>[2x]GWLDLAPSTQVDTETSINVLSDIEFTLNGIYSTMQSSDAYSGRLVYYGDVTGDDMQAVSSTKRTGNYYRFNF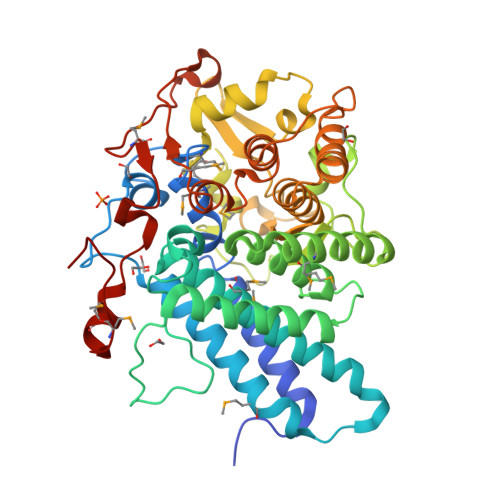TKDNGPSSHWSYLYSIIQNCNLILMNVDKLSIDEDETEYKNDLKGQALAIRGMALFDLTRIFGYPYLKDNGASLGVPIVKELSTIDSKPARNTVAECYTEIISDLKNSTELLSGDFNKGKVNRWAAMTLLSRVYLYKGEYNEALTMAENAIKGAEKEGYALWTNEEYPTAWGNDASASNPGEILFEIVNLTTDSPGKESMGYLNSYNGYDDMCITCSFYQLLKKDPKDVRLKILSFDKKYYAYVNKYQPQQGENITDANIPLIRLSEAYLNAAEAAVQTGDNAKAVKYLNSIVQRANPENSVEGKTLTLENVLDERRKELVAEGHRMYDVIRNGMTVKRIDVKDSDINKTKHNTAYMEYDWNFHKILLPIPKKEMDANPNMKQNPGYVD>GHMDFSQLGGLLDGMKKEFSQLEEKNKDTIHTSKSGGGMVSVSFNGLGELVDLQIDDSLLEDKEAMQIYLMSALNDGYKAVEENRK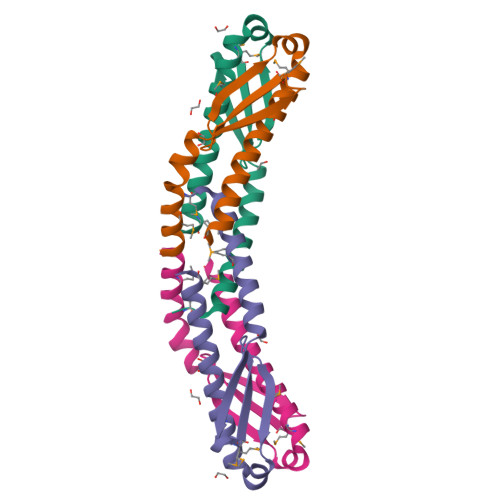NLAFNMLGNFAKL[2x]>MSTVGTGKLTRAQRRAAARKNKRNTRVVQPVIVEPIASGQGKAIKAWTGYSVSKWTASCAAAEAKVTSAITISLPNELSSERNKQLKVGRVLLWLGLLPSVSGTVKSCVTETQTTAAASFQVALAVADNSKDVVAAMYPEAFKGITLEQLAADLTIYLYSSAALTEGDVIVHLEVEH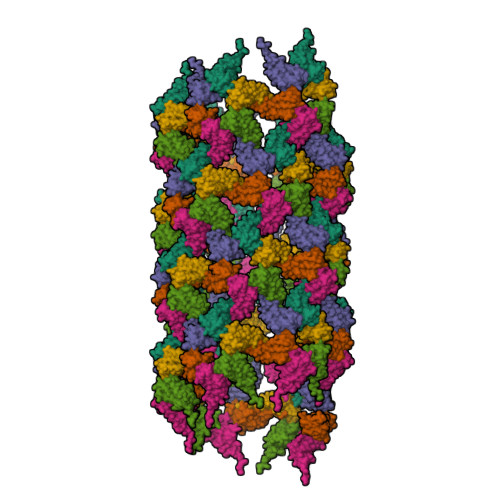VRPTFDDSFTPVY[6x]> GGGMDYAKSDSSSLVTTMGEQFRSLRMLTRRSSPTDVLTGTSVTLPGITIGTDSSLRQSVLNIISYMYRFTKGSISYKIIPKIKGDLYITTSSADNIELNSNAYSFDVNRALHYQNTALNPVVQVSLPYYCPSENLVIDSTSFPNLSNLVLTNLERSSNTYTVLVSAGDDHTFSQLAGCPAFTIGPSRSAA;> MDSSVTNTGGLMPSATISNSEGATMLLNDIPDPTQNVFLSRNVTDNLFEVQDQNLIESLSREVLLGTGTWQSGQAEISTTLTEQQLITNYEQPSIRQISLPDDIVKGSSFIASKLANIAYMRCDYELYLRVQGSPFLQGLLLLWNKMNADQTSKIRSSITEHLRSITSFPGVTLNMQSDSRSVKLVIPYTSEFQVFN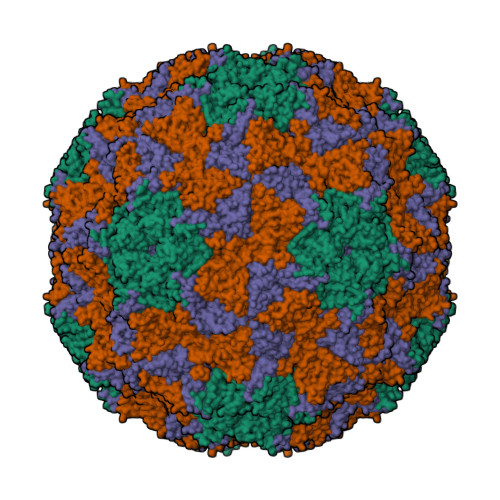PRNENKLNSVRLSILSALRGPSTSEKATYSIMGRMTNIKLYGHAPSIVSLSYPQTE;> SKDRDLSKVSPYENIPAKGFTHGVGFDYGVPLSLFPDNAIDPTIANPESIDEMSIQYLASRPYMLDRYTIKGGNTPSPSGTVVADIPISPVNYSLYGSIIRDYRTIFGAPVSLAVAMASWWRAKIHLNLQFAKTQYHQCRLLVQYLPYGSDVQSLENVLSQIIDISHVDESGIDLCFPSIFTNKWMRSYDPATEGYTAGCAPGRILISVLNPLISASTVNDDIVMMPWLTWENLELAEPGSLAKAAIGFDYPADAVDEKWTSRELPVTGSSFNLFRDTTIVLGASTNISNLVLTNDDTGGDYQIVSTTPTGSYVSAVTCPQGTYTITHDGVGATIISNFPILGAGEGPSFQISALRHGDKVTITEDPTKINVSGVSFLTGTNSWKASLKDSSGTLLGRLEYDGTSFSSDSPASLIPGKYNVELDPADNSAVVTIVANNSFGTASLDTH;> GGDDATASQRGIVTQVADTVSSISNVVDGLGVPLLSSISKPIGWVSNVVSNVASIFGF> MSYYHHHHHHLESTSLYKKAGLENLYFQGDSLLKNEVIKLFNDKPKSGIARIKKWCTDNNQDFIAETAKIFYEEKSNLNLEFVGDYLGTDGVDNQKVLESFTKQFDFKEKDYLESLRRFLQSFKLPGEAQKIDRLVESFGTHYYEQNLNIDINSKDAAYILAYQTIMLNTDLHNPSIAKSKKMTFEQLKNNLKGTNESKNFNDNFLKKIYDEIEAKPFKLNFVKTSPGYELTSTTLNKDSTFKKLDSFLHSTDVNINTVFPGIGDNVKTTVDQPKSWLSFFTGYKGTITLTDNKTSAQATIQVYTPNIFSKWLFGEQPRVIIQPGQTKESIDLAAKAAADFSSPVKNFKATY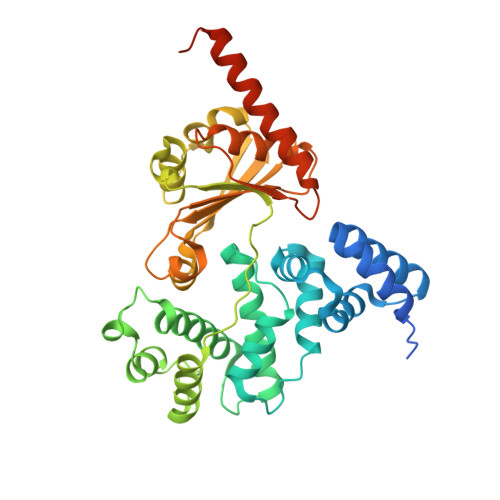DYEVGDLIKAYDNQKKLITIERNLALKEGVPKDPDAEMQKEKGRQLKF> MGASQESELDFVPRLSFLPIEWRSIGSAFGLKDKSGAAANGRATFTVRQGVDAAELTSTGRVIDGQADVGASLKLNTLAIGVSASNITFHSGLDDPTAAAAQRSSLIPSLKLTAAKQFKRDNYIAVSYDLKHQKPELSACWTGEAGADRATLLVNVDPVMRSVKLAAAVRTPGPEWRKVLYNDETDLLEYPADDGARHTLYVQHEV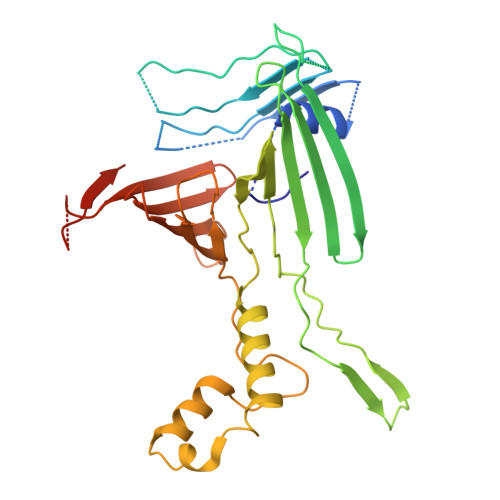RGRDLLHATRLGCRLDLGRLVNYVVDFVDYRIEENIPSFVWNVPLLPQLYSLLVPADNDEQVRHRITGWELDVSHDFARSGLLPVVAISKTSKKLLGGGTLTASYDAAAREAGVSLSRKGVSVGARVARAEGAAGGLSAGWGRPSIHVAVEPLGLLQ>SNVPHKSSLPEGIAPGTVLAIRGLVPPNASRFHVNLLCG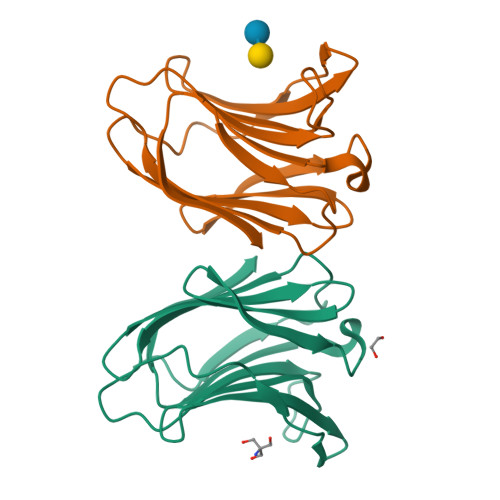EEQGSDAALHFNPRLDTSEVVFNSKEQGSWGREERGPGVPFQRGQPFEVLIIASDDGFKAVVGDAQYHHFRHRLPLARVRLVEVGGDVQLDSVRIF[2x]> AVEPKEDTITVTAAPAPQESAWGPAATIAARQSATGTKTDTPIQKVPQSISVVTAEEMALHQPKSVKEALSYTPGVSVGTRGASNTYDHLIIRGFAAEGQSQNNYLNGLKLQGNFYNDAVIDPYMLERAEIMRGPVSVLYGKSSPGGLLNMVSKRPTTEPLKEVQFKAGTDSLFQTGFDFSDSLDDDGVYSYRLTGLARSANAQQKGSEEQRYAIAPAFTWRPDDKTNFTFLSYFQNEPETGYYGWLPKEGTVEPLPNGKRLPTDFNEGAKNNTYSRNEKMVGYSFDHEFNDTFTVRQNLRFAENKTSQNSVYGYGVCSDPANAYSKQCAALAPADKGHYLARKYVVDDEKLQNFSVDTQLQSKFATGDIDHTLLTGVDFMRMRNDINAWFGYDDSVPLLNLYNPVNTDFDFNAKDPANSGPYRILNKQKQTGVYVQDQAQWDKVLVTLGGRYDWADQESLNRVAGTTDKRDDKQFTWRGGVNYLFDNGVTPYFSYSESFEPSSQVGKDGNIFAPSKGKQYEVGVKYVPEDRPIVVTGAVYNLTKTNNLMADPEGSFFSVEGGEIRARGVEIEAKAALSASVNVVGSYTYTDAEYTTDTTYKGNTPAQVPKHMASLWADYTFFDGPLSGLTLGTGGRYTGSSYGDPANSFKVGSYTVVDALVRYDLARVGMAGSNVALHVNNLFDREYVASCFNTYGCFWGAERQVVATATFRF;> MSFFAGKLNNKSILSLRRGSGGDTNQHINPDSQTIFHSDMSHVIITETHSTGLRLDQGAGDYYWSEMPSRVTQLHNNDPNRVVLTEIEFSDGSRHMLSGMSMGVGAKAYGIINPQIMSQGGLKTQITASADLSLDVGYFNTGTSGTIPQKLRDGTGCQHMFGAFSGRRGFASSAMYLGGAALYKSAWSGSGYVVADAGTLTIPSDYVRHPGARNFGFNAIYVRGRSCNRVLYGMEGPNYTTGGAVQGASSSGALNFTYNPSNPESPKYSVGFARADPTNYAYWESMGDPNDSANGPIGIYSEHLGIYPSKITWYVTNLVYNGSGYNIDGGLFNGNDIKLSPREFIIKGV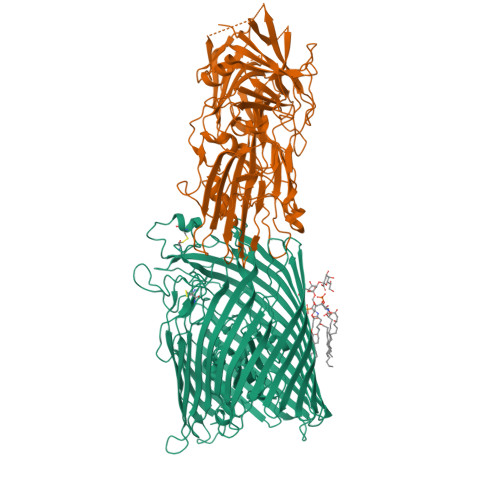NVNNTSWKFINFIEKNFNVGNRADFRDVGCNLSKDSPSTGISGIATFGLPTTESNNAPSIKGGNVGGLHANVVSIYNFLPSASWYVSSNPPKIGNNYGDVWSENLLPLRLLGGSGSTILSGNIVFQGNGSVHVGTVGLDLNSSRNGAIVCTMEFIDDTWLSAGGIGCFNPTEMLSQGAEYGDSRFRIGGNTINKKLHQILSLPAGEYVPFFTIKGTVVNACKLQAAAYNPTPYWVSGLPGSVGQTGYYTLTYYMRNDGNNNISIWLDSSMSNIIGMKACLPNIKLIIQRLTHHHHHH4-METHYL VALERIC ACID | C6 H12 O2 | 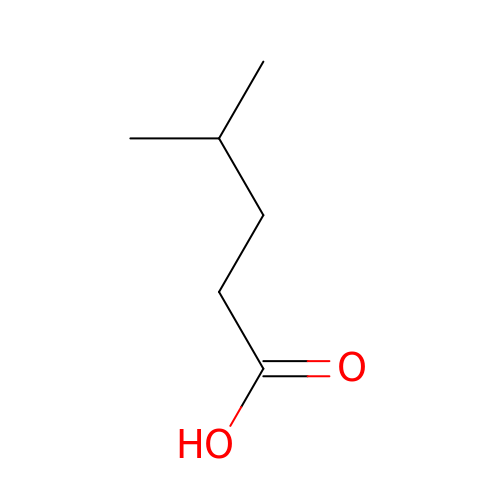FGKJLKRYENPLQH-UHFFFAOYSA-N>[6x]MHADSAPSTTSSQAYAPDARNDAVLVYVNGQFVPRHQAVVSVFDAGYVCGDGVWEGVRLVDGRIVSFDAHIDRMYEGAKSIALDIGMTRAQTKQVVVDTFLRNGMRDGAHARLMVTRGVKKTPNQDPRFIIGGATVVCVAEHKVVTPEAKRNGLKLFTST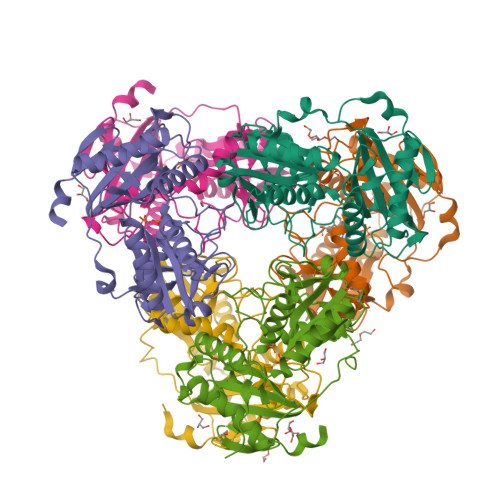LRCSGPDVFDLRLNSHSRLNLIQALIQAIQAGADEALMLDPNGFVSSCNSTNFFAVRNGALWTSSGRYCFNGITRATVVRLAREAGIPVHEGDFTLAEVYAADEAFVTGTLAGLTPVSSVDGRALVPLGPLTQRLDALYRAYIASANEAHGALPAAA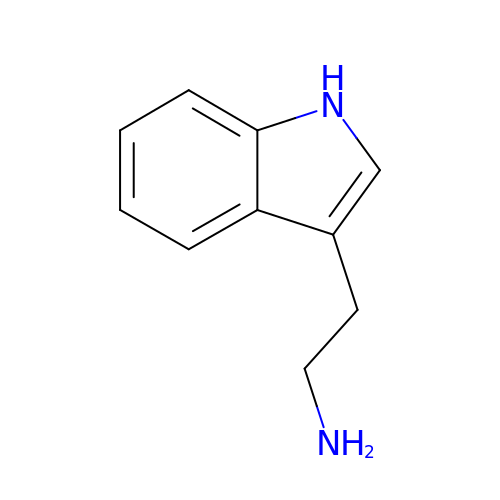2-(1H-INDOL-3-YL)ETHANAMINE | C10 H12 N2 | APJYDQYYACXCRM-UHFFFAOYSA-N> MASWSHPQFEKGASTSLYKKAGLMDSQRSTLVHWFRKGLRLHDNPALSHIFTAANAAPGRYFVRPIFILDPGILDWMQVGANRWRFLQQTLEDLDNQLRKLNSRLFVVRGKPAEVFPRIFKSWRVEMLTFETDIEPYSVTRDAAVQKLAKAEGVRVETHCSHTIYNPELVIAKNLGKAPITYQKFLGIVEQLKVPKVLGVPEKLKNMPTPPKDEVEQKDSAAYDCPTMKQLVKRPEELGPNKFPGGETEALRRMEESLKDEIWVARFEKPNTAPNSLEPSTTVLSPYLKFGCLSARLFNQKLKEIIKRQPKHSQPPVSLIGQLMWREFYYTVAAAEPNFDRMLGNVYCMQIPWQEHPDHLEAWTHGRTGYPFIDAIMRQLRQEGWIHHLARHAVACFLTRGDLWISWEEGQRVFEQLLLDQDWALNAGNWMWLSASAFFHQYFRVYSPVAFGKKTDPQGHYIRKYVPELSKYPAGCIYEPWKASLVDQRAYGCVLGTDYPHRIVKHEVVHKENIKRMGAAYKVNREVRTGKEEESSFE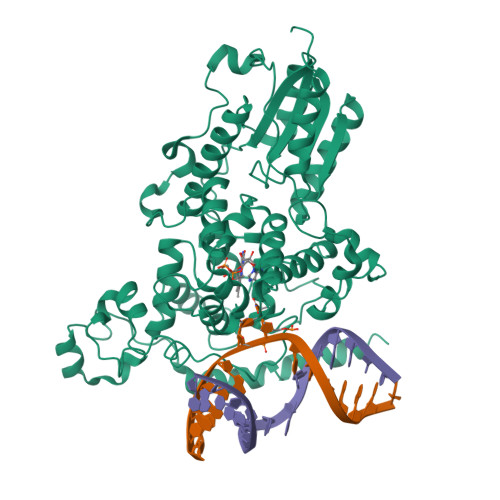EKSET>[2x]STAGKVIKCKAAVLWEVKKPFSIEDVEVAPPKAYEVRIKMVAVGICRTDDHVVSGNLVTPLPVILGHEAAGIVESVGEGVTTVKPGDKVIPLFTPQCGK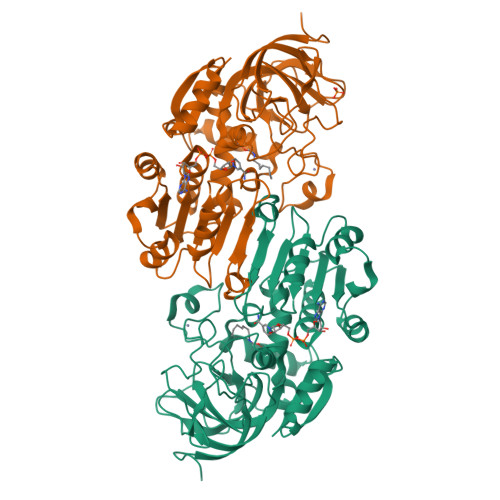CRVCKNPESNYCLKNDLGNPRGTLQDGTRRFTCRGKPIHHFLGTSTFSQYTVVDENAVAKIDAASPLEKVCLIGCGFSTGYGSAVNVAKVTPGSTCAVFGLGGVGLSAVMGCKAAGAARIIAVDINKDKFAKAKELGATECINPQDYKKPIQEVLKEMTDGGVDFSFEVIGRLDTMMASLLCCHEACGTSVIVGVPPASQNLSINPMLLLTGRTWKGAVYGGFKSKEGIPKLVADFMAKKFSLDALITHVLPFEKINEGFDLLHSGKSIRTVLTF>[2x]MSIKIRDFGLGSDLISLTNKAGVTISFTNLGARIVDWQKDGKHLILGFDSAKEYLEKDAYPGATVGPTAGRIKDGLVKISGKDYILNQNEGPQTLHGGEESIHTKLWTYEVTDLGAEVQVKFSLVSNDGTNGYPGKIEMSVTHSFDDDNKWKIHYEAISDKDTVFNPTGHVYFNLNGDASESVENHGLRLAASRFVPLKDQTEIVRGDIVDIKNTDLDFRQEKQ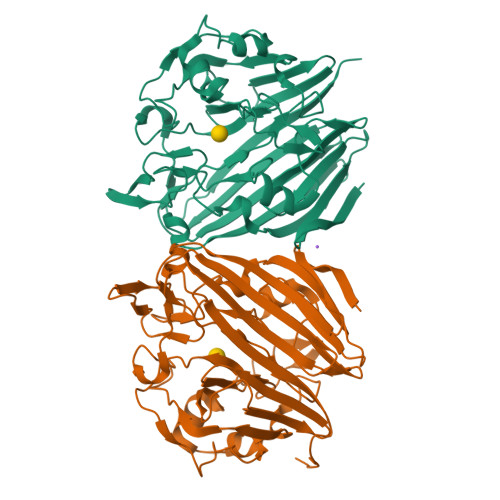LSNAFNSNMEQVQLVKGIAHPFLLDQLGLDKEQARLTLDDTSISVFTDQPSIVIFTANFGDLGTLYHEKKQVHHGGITFECQVSPGSEQIPELGDISLKAGEKYQATTIYSLHTKLEHHHHHH1-(4-{[2-(4-{(4P)-4-[2-amino-4-(difluoromethyl)pyrimidin-5-yl]-6-[(3S)-3-methylmorpholin-4-yl]-1,3,5-triazin-2-yl}piperazin-1-yl)-2-oxoethoxy]methyl}piperidin-1-yl)prop-2-en-1-one | C28 H38 F2 N10 O4 | 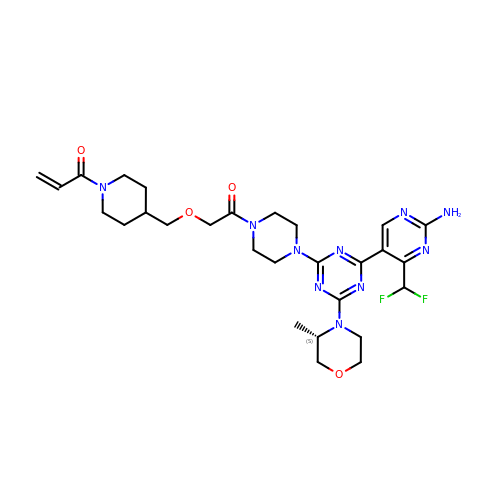PVVOFYPFCTWUAT-SFHVURJKSA-N>[16x]MGVHTFEEESTSP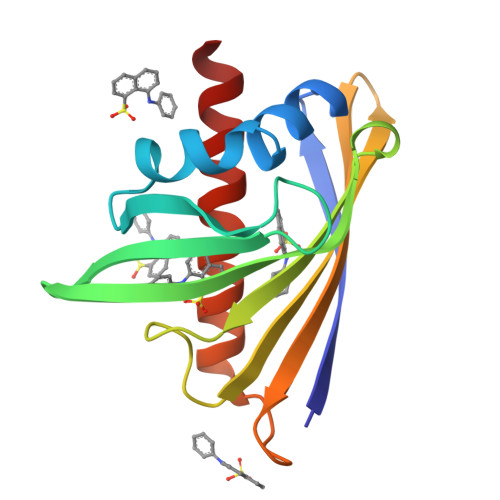VPPAKLFKATVVDGDELTPKLIPAIQSIEIVEGNGGPGTVKKVTAVEDGKTSYVLHKIDAIDEATYTYDYTISGGTGFQEILEKVSFKTKLEAADGGSKIKVSVTFHTKGDAPLPDEVHQDVKQKSQGIFKAIEGYVLSN[(3S)-4-hydroxy-3-{[(4-oxo-4,5-dihydro-3H-pyrrolo[3,2-d]pyrimidin-7-yl)methyl]amino}butyl]phosphonic 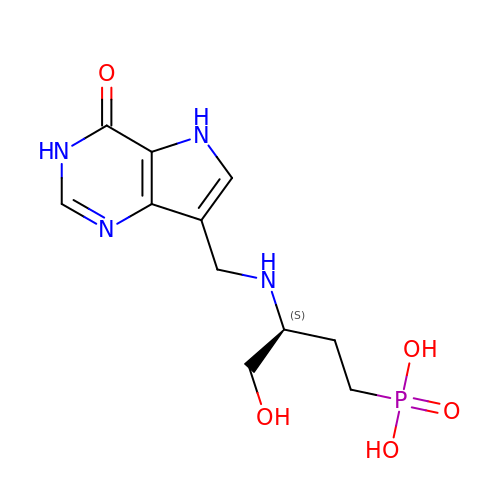acid | C11 H17 N4 O5 P | YYXVNWBGVIIBOW-QMMMGPOBSA-N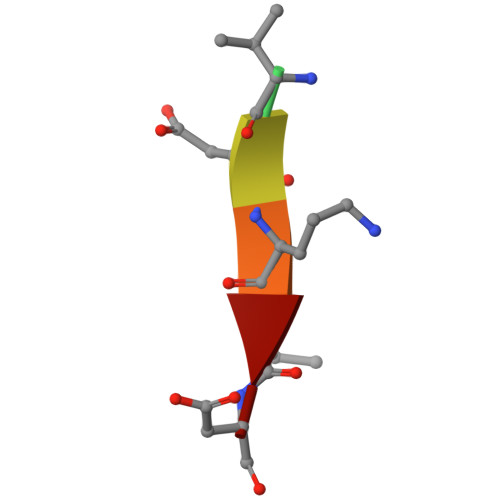> XVDAVD> QDSRGCARWCPQNSSCVNATACRCNPGFSSFSEIITTPTETCDDINECATPSKVSCGKFSDCWNTEGSYDCVCSPGYEPVSGAKTFKNESENTCQDVDE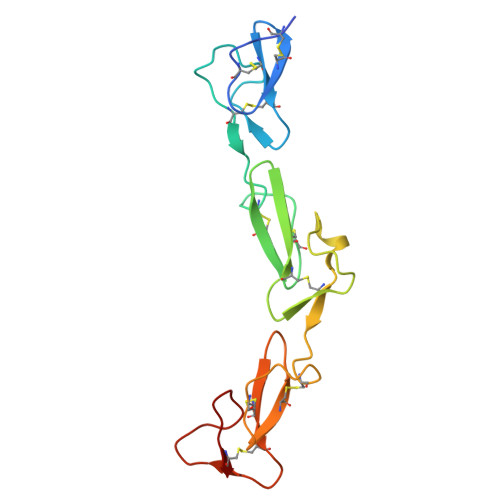CSSGQHQCDSSTVCFNTVGSYSCRCRPGWKPRHGIPNNQKDTVCED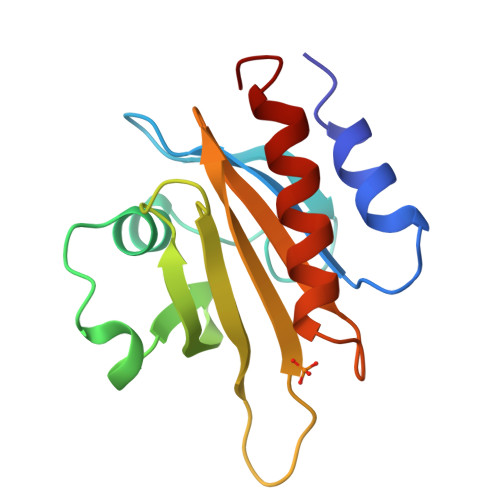> AGWNAYIDNLMADGTCQDAAIVGYKDSPSVWAAVPGKTFVNITPAEVGVLVGKDRSSFYVNGLTLGGQKCSVIRDSLLQDGEFSMDLRTKSTGGAPTFNVTVTKTDKTLVLLMGKEGVHGGLINKKCYEMASHLRRSQY>[28x]G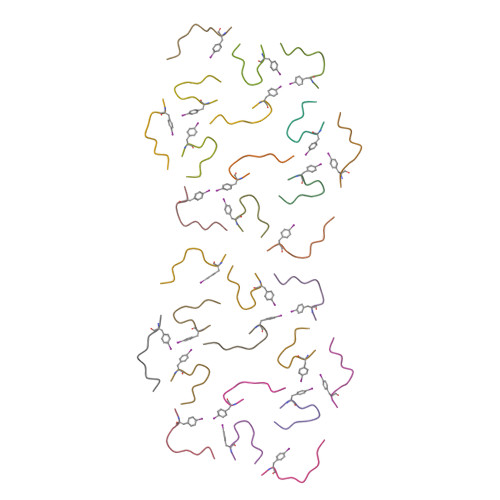FGGNDNFG>MSTFRLALIQLQVSSIKSDNLTRACSLVREAAKQGANIVSLPECFNSPYGTTYF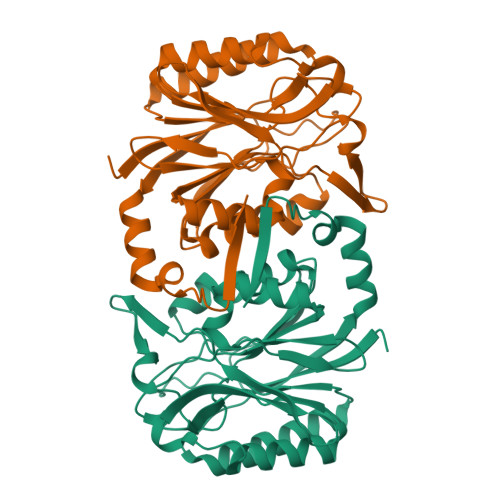PDYAEKIPGESTQKLSEVAKESSIYLIGGSIPEEDAGKLYNTCSVFGPDGSLLVKHRKIHLFDIDVPGKITFQESKTLSPGDSFSTFDTPYCKVGLGICYDMRFAELAQIYAQRGCQLLVYPGAFNLTTGPAHWELLQRARAVDNQVYVATASPARDDKASYVAWGHSTVVDPWGQVLTKAGTEETILYSDIDLKKLAEIRQQIPILKQKRADLYTVESKKP[2x]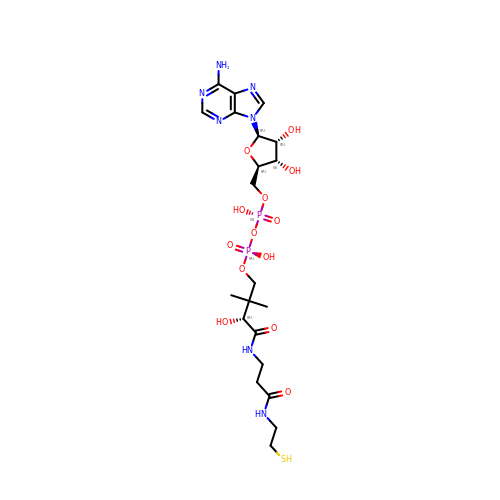DEPHOSPHO COENZYME A | C21 H35 N7 O13 P2 S | KDTSHFARGAKYJN-IBOSZNHHSA-N> MSASQSAVRSRAEAVKVSRTFDYMILFTVFFVVLGGYHIHYMLTGGDWDFWTDWKDRRLWVTVAPIVSITFPAAVQAVLWWRYRIAWGATLCVLGLLLGEWINRYFNFWGWTYFPVNFVFPSNLMPGAIVLDVILMLSNSMTLTAVVGGLAWGLLFYPGNWPIIAPLHVPVEYNGMMMTLADLQGYHYVR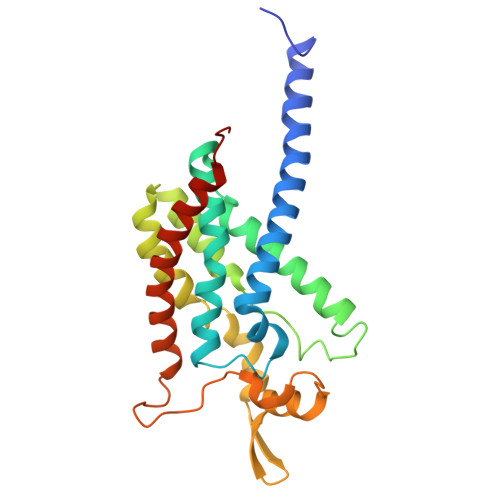TGTPEYIRMVEKGTLRTFGKDVAPVSAFFSGFVSILIYFLWHFFGSWFGSEKFVQAA>[10x]GCCGUCUCAAUAGUGGCUUAGCACAGAUAAUCCAUAGCGAUAUGGGAAAGCUUUUGUAGGUGUAUCAACAAGAGCGCCAGUGAUGGUCAAUCUAAGCAAACCAAUCUUUAUGUAAUCAGUAAUGGUUACAGCACACGAAGUCAAAGCGCAAUACCAGAGCCAAUCGGUGAGGUGCUGUGUCAGCAGUACGUGCGACGAGUGUGUAGGAGGUAUAAACUGACGAAGUUCAAGGGUGGUACCAAGAGCGGUCAGCAUGUUGUGCAACGCUGGGAGGAUAUCCCAGUCAAACACAACAAGUCAAGGUGUACCAGCACCGAGAUAACAAGUAGGCGUUGCGCAUUUUGUUGCUCAAAAGGCGACGAAACGCAAGGCAAUGCACGUCUGCGAUACACGAAAACAAUGCUAUUUGUUGAAAAUAUUGGAAUAA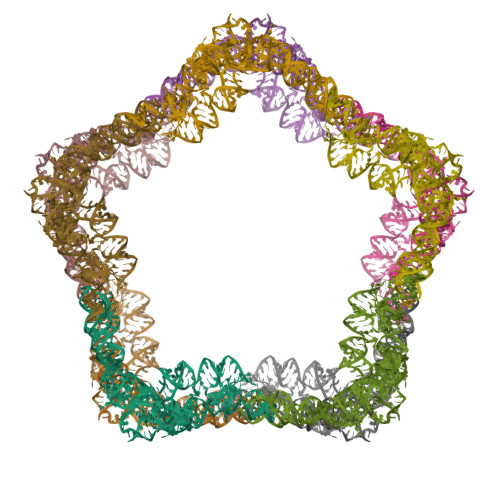AGCAAAAGUCAUUGCCCGUCGCAAACGAAAGUGUGCUUCGGUAGCUAGGCUACCUGCUAGAGUCUCGCAAGGAUAAUAGCAAAGUCAAAGAGUAAAGCAGCUUAGACCUUUAGCGGGGUUUUCGUUAAUUGAAAAAUGGCUUAGUAGUUUGCGGCGUAACGAGUGGUUAGCGAUACUAACCGCGCAUGGUUGUUACUUGAAGGGAUUUGAGUGGAUAAAAAACUAAAACAUAAGGUUUUGAAAGACAACUGACUAAACGUGUAAUCUCAGCGU> MPFIEC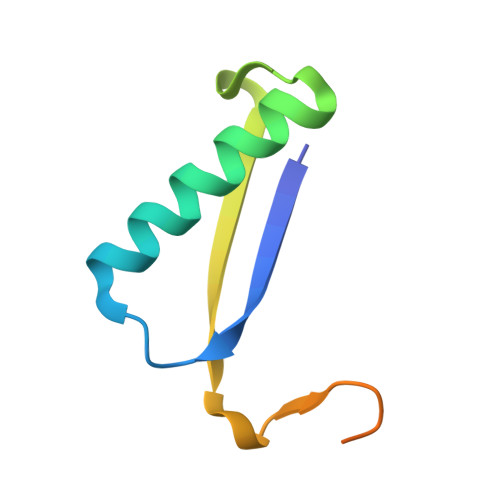HIATGLSVARKQQLIRDVIDVTNKSIGSDPKIINVLLVEHAEANMSISGRIHGEAASTERTPAVS>[3x]SSPPVVDTVHGKVLGKFVSLEGFAQPVAIFLGIPFAKPPLGPLRFTPPQPAEPWSFVKNATSYPPMCTQDPKAGQLLSELFTNRKENIPLKLSEDCLYLNIYTPADLTKKNRLPVMVWIHGGGLMVGAASTYDGLALAAHENVVVVTIQYRLGIWGFFSTGDEHSRGNWGHLDQVAALRWVQDNIASFGGNPGSVTIFGESAGGESVSVLVLSPLAKNLFHRAIS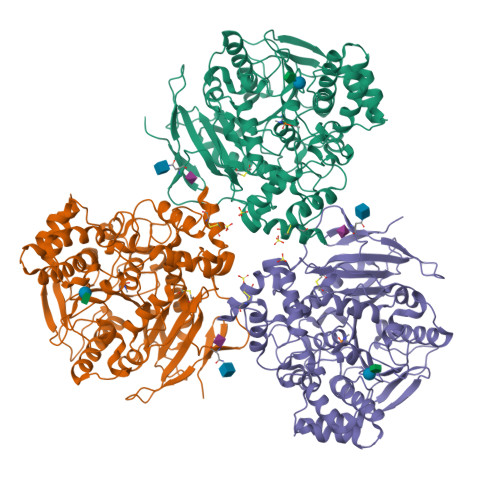ESGVALTSVLVKKGDVKPLAEQIAITAGCKTTTSAVMVHCLRQKTEEELLETTLKMKFLSLDLQGDPRESQPLLGTVIDGMLLLKTPEELQAERNFHTVPYMVGINKQEFGWLIPMLMSYPLSEGQLDQKTAMSLLWKSYPLVCIAKELIPEATEKYLGGTDDTVKKKDLFLDLIADVMFGVPSVIVARNHRDAGAPTYMYEFQYRPSFSSDMKPKTVIGDHGDELFSVFGAPFLKEGASEEEIRLSKMVMKFWANFARNGNPNGEGLPHWPEYNQKEGYLQIGANTQAAQKLKDKEVAFWTNLFAK>LYDMNGCYSRLKELVPTLPQNRKVSKVEILQ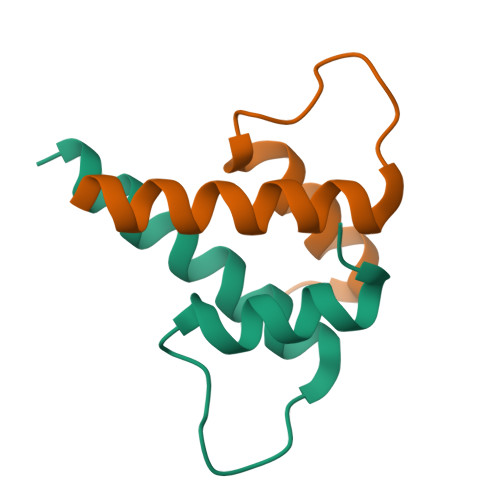HVIDYIRDLQLELNS[2x]Carboxylesterases (EC 3.1.1.1.) and lipases (EC 3.1.1.3) catalyse the hydrolysis and synthesis of ester bonds across a large variety of substrates. Esterases generally show promiscuous activity with a specificity for either the alcohol or acid moiety. They are members of the α/β hydrolase superfamily with most using a catalytic triad of serine, aspartic acid and histidine in the active site, where the serine residue (found in the sequence motif GxSxG), is responsible for the nucleophilic attack on the substrate. We have described seven members of a new family of serine esterases all containing a C-terminal OsmC-like domain taken from extremophilic bacteria from a wide range of ecological niches. An enzyme from the thermophilic bacterium, Rhodothermus marinus showed particularly high activity, even at low temperatures and was subjected to further kinetic characterisation and crystal structure determination.

While the full length OsmC esterases were recalcitrant to our attempts at structure determination, the putative esterase from Rhodothermus marinus, EstRM, was crystallised as a C-terminal truncation comprising residues 1–255 of the 410 amino acid full-length protein, including the alpha-beta-hydrolase domain, with a C-terminal hexa-histidine tag. The structure was determined by molecular replacement to 1.56 Å resolution. The structure consists of two molecules in the asymmetric unit, which align with an rmsd of 0.35 Å in their Cα positions over 225 residues and can thus be considered identical in their overall fold. Molecule A has visible electron density for residues 1–70, 82–150, and 153–253; while molecule B has visible electron density for residues 2–70, 84–148, 156–168, 175–253. ΔEstRM has a classical α/β-hydrolase fold, with a core β-sheet made up of seven parallel strands (β1, β3–6, β10–11) and one antiparallel strand (β2); one face of the protein is flanked by two alpha helices (α1 and 8) and the other by four helices (α2, 3, 6, 7). There is an insertion in the α/β hydrolase fold between β6 and α6, which is formed by α4, β7, β8, β9, and α5, encompassing residues 136–180. The inserted domain between β6 and α6 forms a lid that completely occludes the active site, with a loop formed by residues 160–165 sitting directly above S109. The differences seen between the two chains in the asymmetric unit and high B-factors indicate that the lid region is likely to be flexible and may act to modulate the accessibility of the active site. The structure of ΔEstRM has a partially occupied intra-molecular disulphide bond between residues C135 and C210. This disulphide links α7 with the loop preceding α4, stabilising the position of the beginning of the insertion domain.

>[2x]MQIKTVTFENNRGERLAARLDLPVDTQPVAYALFAHCFTCSKNLKAVTTISRALTTQGYAVLRFDFTGLGESEGDFSETTFATNFEDLRAACRFLSAQYEPPALLIGHSLGGAAVLAVAGEFPEVKAVATIGAPCDPAHVRHLLRPALDTIKTVGEAVVDLGGRPFRIKKQFLEELERVNLEDQVRTMRRPLLLFHSPTDQIVGIENAACLFQAARHPKSFVSLDQADHLLSNSDDAAFVGEVLGAWARRYVGRRLGHHHHHH>[2x]SNAMKDILRD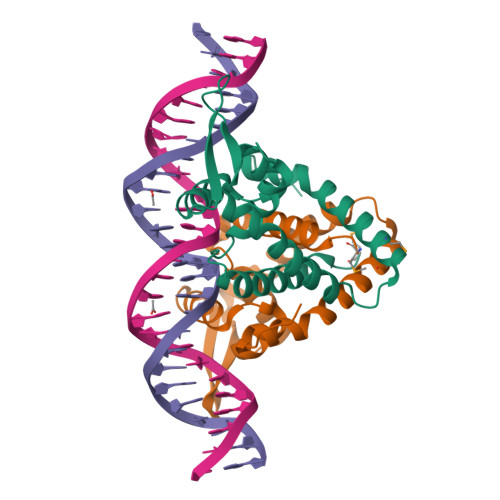IGVIARALDSISNIEFKELNLAKGQFIYLVRICENQGIIQEKLVDILKIDRTTASRAIKNLEKNGLIIKKQNKNNKKNKLLFPTEKGQQLYPLIIRENEYSNAVALKGFTEAEINMLTDALKKVKENIADDWLYVKKGNKRSY> MEKMHITNQEHDAFVKSHPNGDLLQLTKWAETKKLTGWYARRIAVGRDGEVQGVAQLLFKKVPKLPYTLCYISRGFVVDYSNKEALNALLDSAKEIAKAEKAYAIKIDPDVEVDKGTDALQNLKALGFKHKGFKEGLSKDYIQPRMTM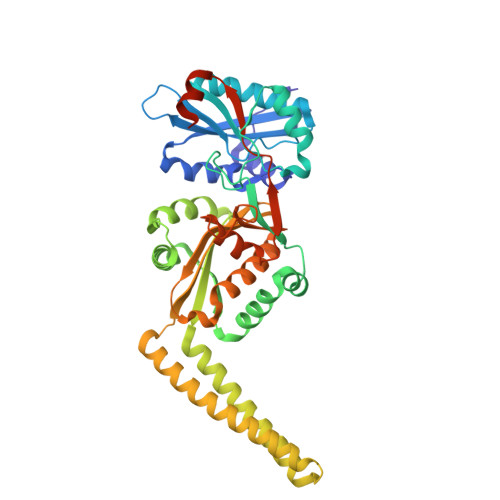ITPIDKNDDELLNSFERRNRSKVRLALKRGTTVERSDREGLKTFAELMKITGERDGFLTRDISYFENIYDALHEDGDAELFLVKLDPKENIAKVNQELNELHAEIAKWQQKMETSEKQAKKAQNMINDAQNKIAKNEDLKRDLEALEKEHPEGIYLSGALLMFAGSKSYYLYGASSNEFRDFLPNHHMQYTMMKYAREHGATTYDFGGTDNDPDKDSEHYGLWAFKKVWGTYLSEKIGEFDYILNQPLYQLIEQVKPRLTKAKIKISRKLKR>ETPSQKCEEKYKGNTDKISCLHHCKYQYYGFIDVNYNIAQSEIRKFSNVLMDYGVVDKSKKRELKKVMHECAKQVKKEARKDSHWLNCRTSINYYRCVLTSKLIGPQRFDKAIQD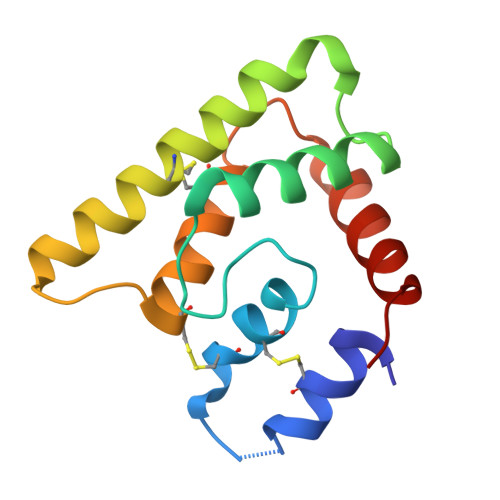YDKTISV[7x]ClfB, an MSCRAMM (Microbial Surface Components Recognizing Adhesive Matrix Molecules) family surface protein, described as a fibrinogen-binding clumping factor, is a key determinant of S. aureus nasal colonization, but the molecular basis for ClfB-ligand recognition remains unknown. ClfB plays a key role in establishing human nasal colonization by binding to the human type I cytokeratin 10 (CK10) expressed on squamous epithelial cells. As a bifunctional MSCRAMM, ClfB also binds to fibrinogen α (Fg α), which is assumed to be significant in platelet activation and aggregation and has been shown to contribute to the pathogenesis of experimental endocarditis in rats. In this study, we solved the crystal structures of apo-ClfB and its complexes with fibrinogen α (Fg α) and cytokeratin 10 (CK10) peptides.

The apo-ClfB(197–534) structure was solved at 2.5 Å resolution, consisting of residues Ser197-Ala534. No electron density was observed for the C-terminal eight residues in the apo-ClfB structure. The polypeptide chain of apo-ClfB(197–534) is composed of two distinct domains N2 and N3, as previously described for other MSCRAMMs in S. aureus. The N-terminal N2-domain contains 146 residues (amino acids 213–358) and the N3 domain 170 residues (amino acids 359–528). In the crystal structure, both N2 and N3 have two layers of β-sheets that pack tightly against each other. In contrast, packing between the two domains is much looser, resulting in the formation of a large groove between them where presumably ligands bind. In the crystal structure of apo-ClfB, the N-terminus (Ser197-Ala201) of one ClfB(197–542) molecule binds to the N3 domain of a symmetry-related ClfB molecule, forming a β-sheet together with the strand G mediated by 2 pairs of main-chain hydrogen bonds. Additional hydrogen bonds involving ClfBGln235 and ClfBVal200 further contribute to the N-terminus-mediated interaction between ClfBs. These interactions may act together to stabilize the G-strand of the N3 domain, thus maintaining its Dev-IgG fold and mimicking the transition state of ligand binding. Structural comparison of the apo-ClfB and the two complexes shows that the RMSDs of the Cα atoms in ClfB are 0.46 Å and 0.49 Å respectively, indicating that the overall ClfB remains unchanged upon binding of the ligands.

> MRGSHHHHHHENLYFQGSLAVAEPVVNAADAKGTNVNDKVTASDFKLEKTAFDPNQSGNTFMAANFKVTGQVKSGDYFTAKLPDSVTGNGDVDYSNSNNTMPIADIKSTNGDVVAKATYDILTKTYTFVFTDYVNDKENINGQFSLPLFTDRAKAPKSGTYDANINIADEMFDNKITYNYSSPIAGIDKPNGANISSQIIGVDTASGQNTYKQTVFVNPKQRVLGNTWVYIKGYQDKIEESSGKVSATDTKLRIFEVNDTSKLSDSYYADPNDSNLKEVTGEFKDKISYKYDNVASINFGDINKTYVVLVEGHYDNTGKNLKTQVIQENIDPATGKDYSIFGWNNENVVRYGGGSADGDSAVN> GEIQWVKPNKETGRLNINGPTRTKLEPSVFHDIFEGNKEPAVLHSKDPRLEVDFEQALFSKYVGNTLHEPDEYIKEAALHYANQLKQLEINTSQMSMEEACYGTEN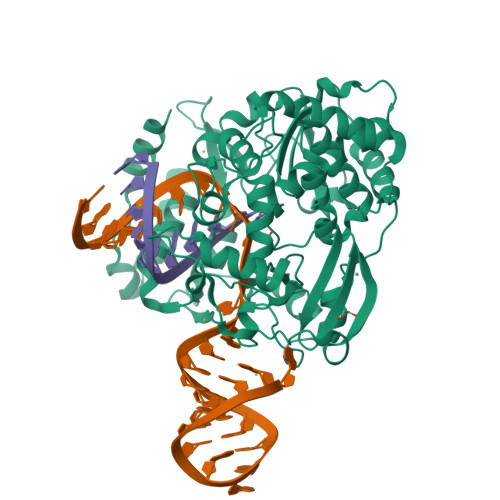LEAIDLHTSAGYPYSALGIKKRDILDPTTRDVSKMKFYMDKYGLDLPYSTYVKDELRSIDKIKKGKSRLIEASSLNDSVYLRMAFGHLYEAFHANPGTITGSAVGCNPDTFWSKLPILLPGSLFAFDYSGYDASLSPVWFRALELVLREIGYSEEAVSLIEGINHTHHVYRNKTYCVLGGMPSGCSGTSIFNSMINNIIIRALLIKTFKGIDLDELNMVAYGDDVLASYPFPIDCLELAKTGKEYGLTMTPADKSPCFNEVNWGNATFLKRGFLPDEQFPFLIHPTMPMREIHESIRWTKDARNTQDHVRSLCLLAWHNGKQEYEKFVSTIRSVPVGRALAIPNYENLRRNWLELFHHHHHH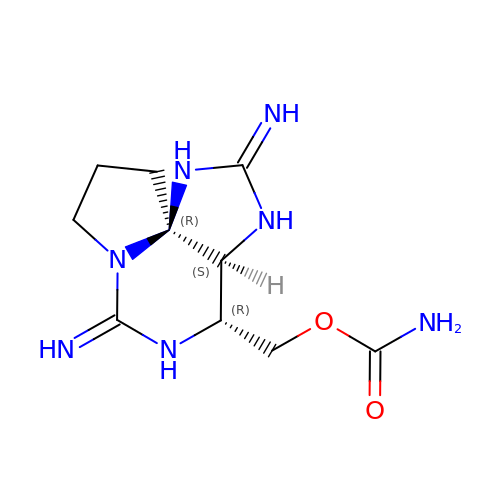[(2Z,3aS,4R,6Z,10aR)-2,6-diiminooctahydro-1H,8H-pyrrolo[1,2-c]purin-4-yl]methyl carbamate | C10 H17 N7 O2 | WSPXQONARWJOKG-JFWOZONXSA-N> GSTRRRTRLRPPTPL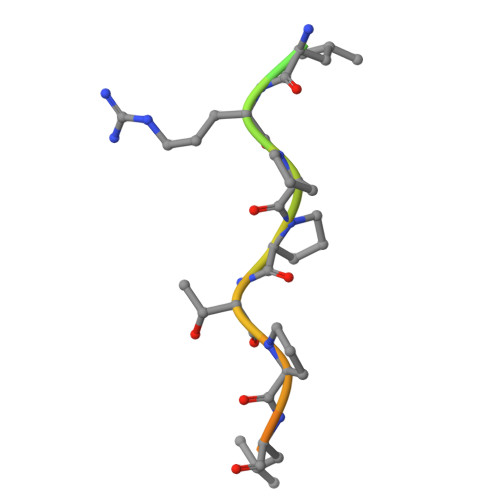SQLLSP>SAAATQAVPAPNQQPEVFCNQIFINNEWHDAVSRKTFPTVNPSTGEVICQVAEGDKEDVDKAVKAARAAFQLGSPWRRMDASHRGRLLNRLADLIERDRTYLAALETLDNGKPYVISYLVDLDMVLKCLRYYAGWADKYHGKTIPIDGDFFSYTRHEPVGVCGQIIPWNFPLLMQAWKLGPALATGNVVVMKVAEQTPLTALYVANLIKEAGFPPGVVNIVPGFGPTAGAAIASHEDVDKVAFTGSTEIGRVIQVAAGSSNLKRVTLELGGKSP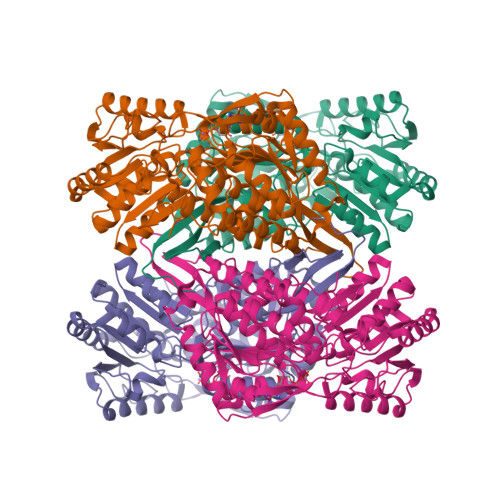NIIMSDADMDWAVEQAHFALFFNQGQCCCAGSRTFVQEDIYDEFVERSVARAKSRVVGNPFDSKTEQGPQVDETQFKKILGYINTGKQEGAKLLCGGGIAADRGYFIQPTVFGDVQDGMTIAKEEIFGPVMQILKFKTIEEVVGRANNSTYGLAAAVFTKDLDKANYLSQALQAGTVWVNCYDVFGAQSPFGGYKMSGSGRELGEYGLQAYTEVKTVTVKVPQKNS[8x]>MPAPQPQPVLAPLTPAAVFLVATIDEGQEATVY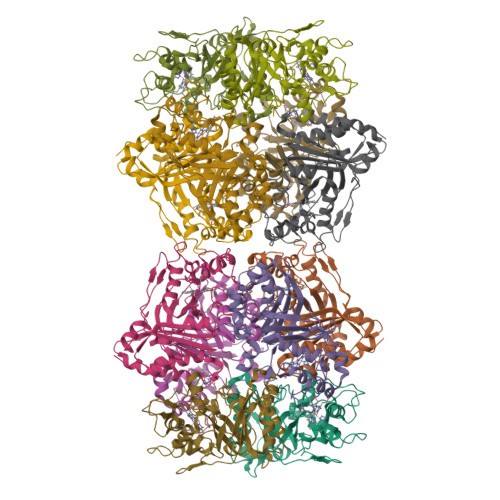DALPDISGLVRAIGFRDPAKRLSAITSIGSDAWDRLFSGPRPAELHPFREIDGGRHHAPATPGDLLFHLRAESMDVCFELATKLVEAMSGAITIVDETHGFRFFDNRDLMGFVDGTENPDGNLAVVATQIGDEDPDFAGGCYVHVQKYLHDMASWNSLSVEEQERVIGRTKLDDIELDDDVKPANSHVALNVIEDEDGNELKIIRHNMPFGEIGKGEFGTYYIGYSRTPSVTERMLDNMFIGDPPGNTDRILDFSTAITGGLFFTPTVDFLDDPPPLPSEDDRAEPASAPSADPVHTDGSLGIGSLKGTR[6x]>MRGSHHHHHHGSMDKNIIIGAMTALITPFKNGKVDEQSYARLIKRQIENGIDAVVPVGTTGESATLTHEEHRTCIEIAVETCKGTKVKVLAGAGSDATHEAVGLAKFAKEHGADGILSVAPYYNKPTQQGLYEHYKAIAQSVDIPVLLYNVPGRTGCEISTDTIIKLFRDCENIYGVKEASGNIDKCVDLLAHE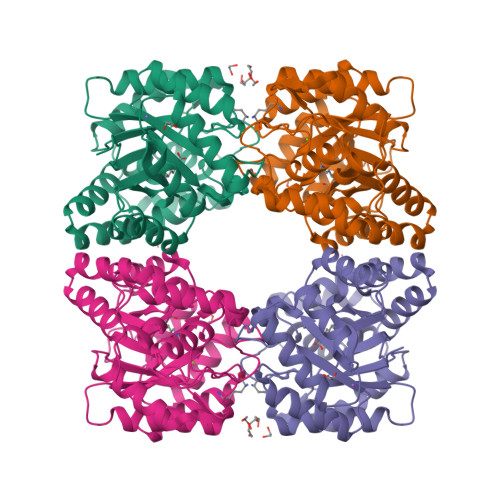PRMMLISGEDAINYPILSNGGKGVISVTSNLLPDMISALTHFALDENYKEAKKINDELYNINKILFCESNPIPIKTAMYLAGLIESLEFRLPLCSPSKENFAKIEEVMKKYKIKGF[6x]> MDHRTSIAQAMVDRISKQMDGSQPDEYFNNLYGNVSRQTYKFEEIREFPYVAVHIGTETGQYLPSGQQWMFLELPILVYDKEKTDIQEQLEKLVADIKTVIDTGGNLEYTVSKPNGSTFPCEATDMIITSVSTDEGLLAPYGLAEIN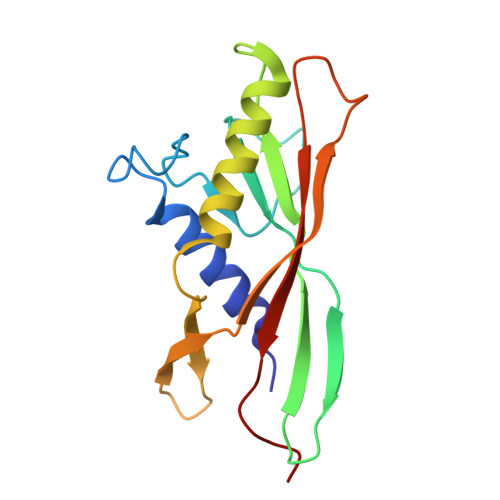VTVRYQPPRRSLRR> SDLEVEKFKQKFISLAKSQDQHGSQEDKSTLFDEEYEFQLLLAEAKLPQLSNNLSSKDPAMKKNYESLNQLQQDLENLLAPFQSVKETEQNWKLRQSNIIELDNIISGNIPKDNPEEFVTVIKEVQLIELISRATSSLRTTLSLTALLFLKRLIHILNDQLPLSILDQIF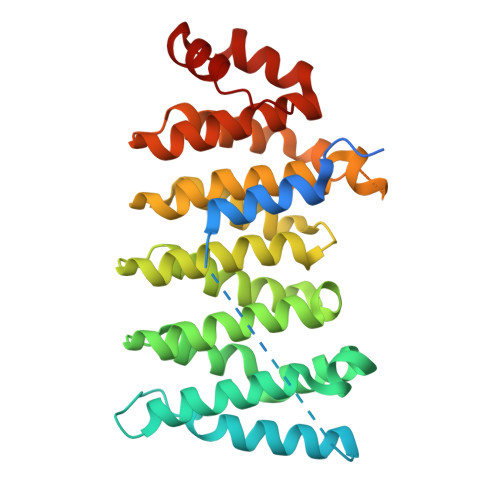VIFKNLLSSTKKISSQTAFHCLITLIIDINHFHNKLFQLSFLLINEKTVTPRFCSAILLRSFLIKFNDSNLSLNNSNTTSPTSKLENNIIYIEEWLKKGISDSQTTVREAMRLTFWYFYKCYPTNAKRLLSSSFSPQLKKATELAIPAHL>[2x]QSASNVRATYHFYNAQQNGWDLRKVSAYCATWDADKPYSWRSKYGWTAFCGPVGPH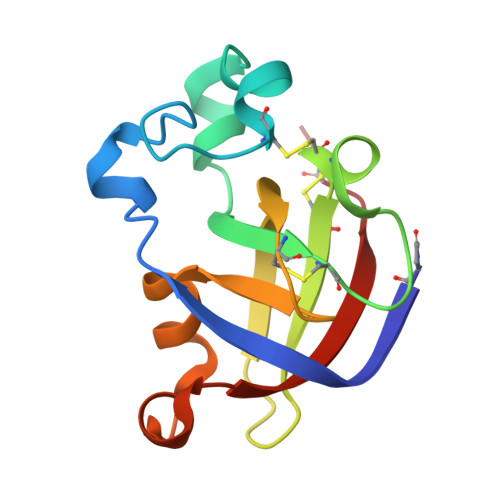GRAACGKCLRVTNTKTRAETTVRIVDQCSNGGLDLDWSVFKKLDTDGSGYLRGHLIVNYQFVNCGN>[2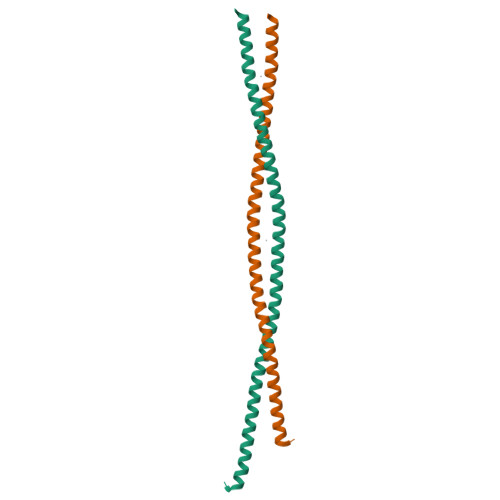x]GSSPLLKSAEREKEMASMKEEFTRLKEALEKSEARRKELEEKMVSLLQEKNDLQLQVQAEQDNLADAEERCDQLIKNKIQLEAKVKEMNERLEDEEEMNAELTAKKRKLEDECSELKRDIDDLELTLAK>[3x]SFVEMVDNLRGKSGQGYYVEMTVGSPPQTLNILVDTGSSNFAVGAAPHPFLH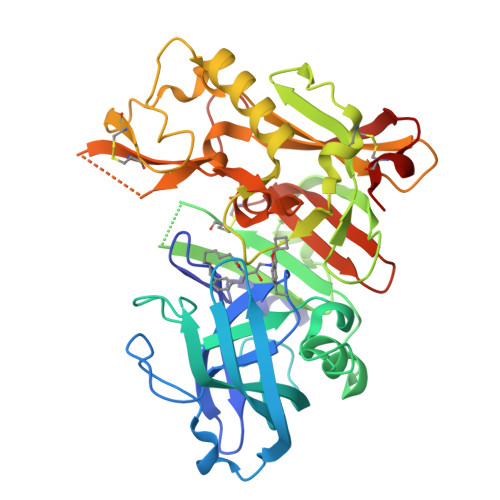RYYQRQLSSTYRDLRKGVYVPYTQGKWEGELGTDLVSIPHGPNVTVRANIAAITESDKFFINGSNWEGILGLAYAEIARPDDSLEPFFDSLVKQTHVPNLFSLQLCGAGFPLNQSEVLASVGGSMIIGGIDHSLYTGSLWYTPIRREWYYEVIIVRVEINGQDLKMDCKEYNYDKSIVDSGTTNLRLPKKVFEAAVKSIKAASSTEKFPDGFWLGEQLVCWQAGTTPWNIFPVISLYLMGEVTNQSFRITILPQQYLRPVEDVATSQDDCYKFAISQSSTGTVMGAVIMEGFYVVFDRARKRIGFAVSACHVHDEFRTAAVEGPFVTLDMEDCGYN>GGMELRVGNRYRLGRKIGSGSFGDIYLGTDIAAGEEVAIKLECVKTK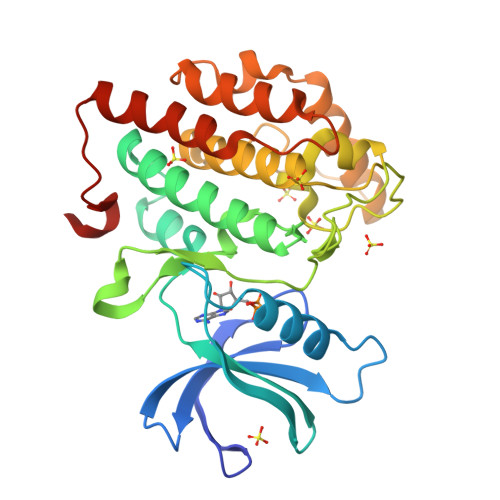HPQLHIESKIYKMMQGGVGIPTIRWCGAEGDYNVMVMELLGPSLEDLFNFCSRKFSLKTVLLLADQMISRIEYIHSKNFIHRDVKPDNFLMGLGKKGNLVYIIDFGLAKKYRDARTHQHIPYRENKNLTGTARYASINTHLGIEQSRRDDLESLGYVLMYFNLGSLPWQGLKAATKRQKYERISEKKMSTPIEVLCKGYPSEFATYLNFCRSLRFDDKPDYSYLRQLFRNLFHRQGFSYDYVFDWNMLK[2x]3-(5,6-dimethyl-2H-isoindol-2-yl)-N'-[(E)-furan-2-ylmethylidene]benzohydrazide 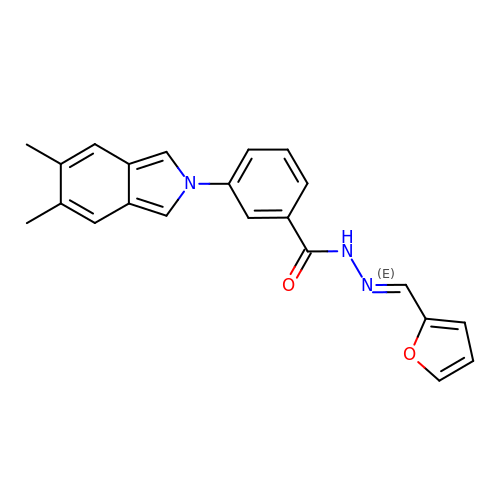| C22 H19 N3 O2 | JOUFONRDAYRIBB-FSJBWODESA-N> GSHMASMNSEILNNIILNLRYKDNNLIDLSGYGAKVEVYDGVELNDKNQFKLTSSANSKIRVTQNQNIIFNSVFLDFSVSFWIRIPKYKNDGIQNYIHN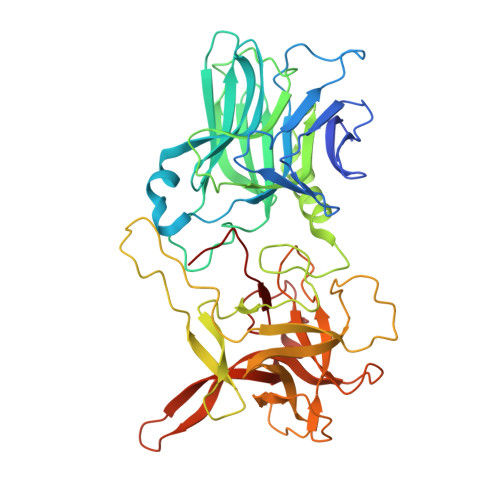EYTIINCMKNNSGWKISIRGNRIIWTLIDINGKTKSVFFEYNIREDISEYINRWFFVTITNNLNNAKIYINGKLESNTDIKDIREVIANGEIIFKLDGDIDRTQFIWMKYFSIFNTELSQSNIEERYKIQSYSEYLKDFWGNPLMYNKEYYMFNAGNKNSYIKLKKDSPVGEILTRSKYNQNSKYINYRDLYIGEKFIIRRKSNSQSINDDIVRKEDYIYLDFFNLNQEWRVYTYKYFKKEEEKLFLAPISDSDEFYNTIQIKEYDEQPTYSCQLLFKKDEESTDEIGLIGIHRFYESGWWFEEYKDYFCISKWYLKEVKRKPYNLKLGCNWQFIPKDEGWTE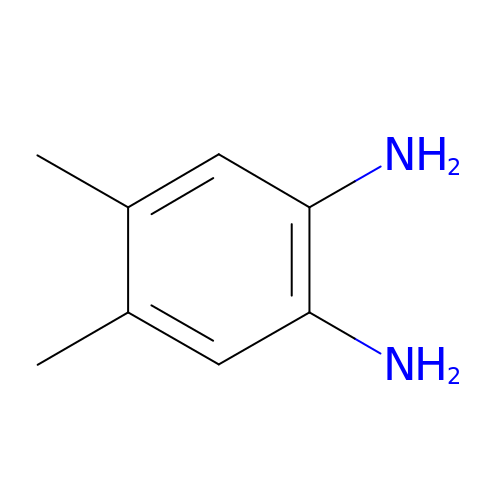4,5-DIMETHYL-1,2-PHENYLENEDIAMINE | C8 H12 N2 | XSZYBMMYQCYIPC-UHFFFAOYSA-N> DNLIYLDLNLQDW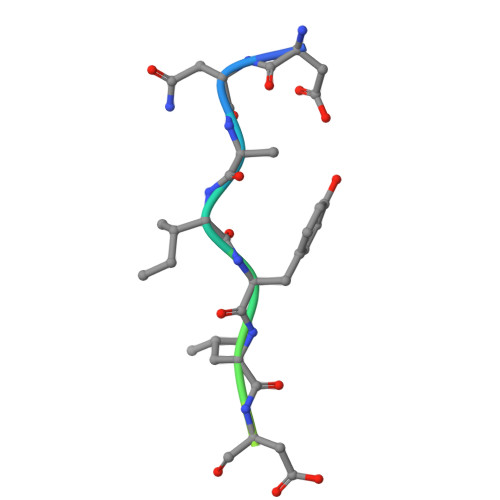DD4-bromanyl-~{N}-methyl-1~{H}-pyrrole-2-carboxamide 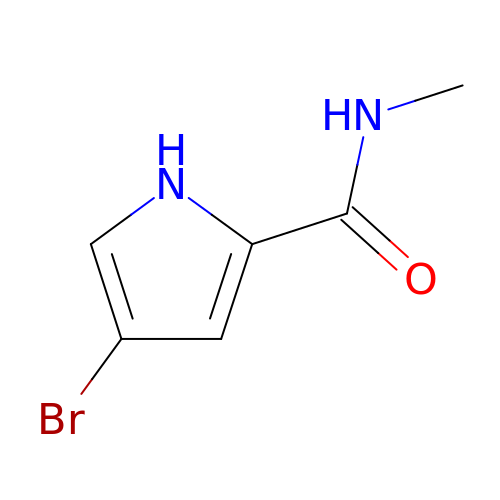| C6 H7 Br N2 O | HQGRBJIXXLIGLE-UHFFFAOYSA-N>PSYVAHLASDFGVRVFQQVAQASKDRNVVFSPYGVASVLAMLQLTTGGETQQQIQAAMGFKIDDKGMAPALRHLYKELMGPWNKDEISTTDAIFVQRDLKLVQGFMPHFFRLFRSTVKQVDFSEVERARFIINDWVKTHTKGMISHLLGTGAVDQLTRLVLVNALYFNGQWKTPFPDSSTHRRLFHKSDGSTVSVPMMAQTNKFNYTEFTTPDGHYYDILELPYHGDTLSMFIAAPYEKEVPLSALTNILSAQLISHWKGNMTRLPRLLVLPKFSLETEVDLRKPLENLGMTDMFRQFQADFTSLSDQEPLHVALALQKVKI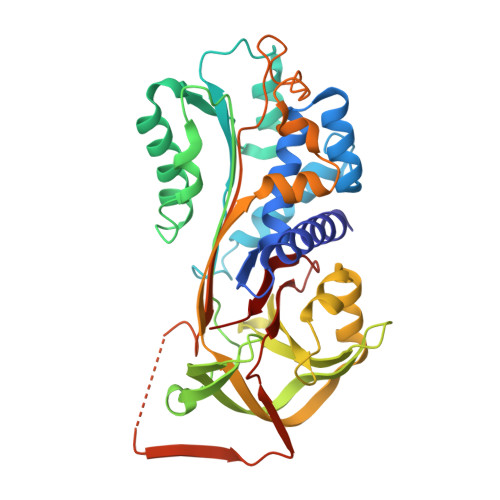EVNESGTVASSSTAVIVSARMAPEEIIIDRPFLFVVRHNPTGTVLFMGQVMEP[4x]> LY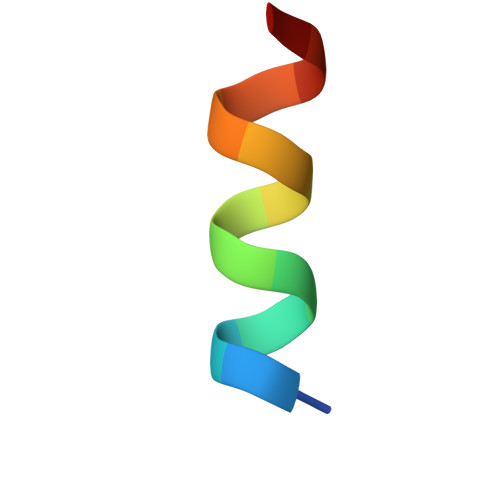KHFLKLFWLALX> VVMSRGRIPRLGAAVLVALTTAAAACGADSQGLVVSFYTPATDGATFTAIAQRCNQQFGGRFTIAQVSLPRSPNEQRLQLARRLTGNDRTLDVMALDVVWTAEFAEAGWALPLSDDPAGLAENDAVADTLPGPLATAGWNHKLYAAPVTTNTQLLWYRPDLVNSPPTDWNAMIAEAARLHAAGEPSWIAVQANQGEGLVVWFNTLLVSAGGSVLSEDGRHVTLTDTPAHRAATVSALQILKSV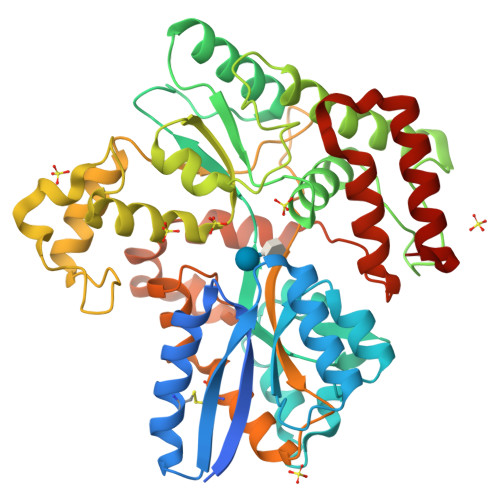ATTPGADPSITRTEEGSARLAFEQGKAALEVNWPFVFASMLENAVKGGVPFLPLNRIPQLAGSINDIGTFTPSDEQFRIAYDASQQVFGFAPYPAVAPGQPAKVTIGGLNLAVAKTTRHRAEAFEAVRCLRDQHNQRYVSLEGGLPAVRASLYSDPQFQAKYPMHAIIRQQLTDAAVRPATPVYQALSIRLAAVLSPITEIDPESTADELAAQAQKAIDGMGLLP> MSMLKREDWYDLTRTTNWTPKYVTENELFPEEMSGARGISMEAWEKYDEPYKITYPEYVSIQREKDSGAYSIKAALERDGFVDRADPGWVSTMQLHFGAIALEEYAASTAEARMARFAKAPGNRNMATFGMMDENRHGQIQLYFPYANVKRSRKWDWAHKAIHTNEWAAIAARSFFDDMMMTRDSVAVSIMLTFAFETGFSNMQFLGLAADAAEAGDHTFASLISSIQTDESRHAQQGGPSLKILVENGKKDEAQQMVDVAIWRSWKLFSVETGPIMDYYTPLESRNQSFKEFMLEWIVAQFERQLLDLGLDKPWYWDQFMQDLDE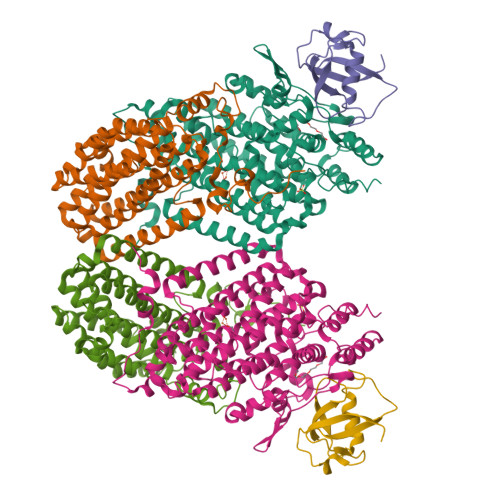THHGMHLGVWYWRPTVWWDPAAGVSPEEREWLEEKYPGWNDTWGQCWDVITDNLVNGKPELTVPETLPTICNMCNLPIAHTPGNKWNVKDYQLEYEGRLYHFGSEADRWCFQIDPERYKNHTNLVDRFLKGEIQPADLAGALMYMSLEPGVMGDDAHDYEWVKAYQKKTNAA;> MSEQQPEALKPLKTWSHLAGNRRRPSEYEVVSTNLHYFTDNPERPWELDSNLPMQTWYKKYCFDSPLKHDDWNAFRDPDQLVYRTYNLLQDGQESYVQGLFDQLNDRGHDQMLTREWVETLARFYTPARYLFHALQMGSVYIHQIAPASTITNCATYETADHLRWLTHTAYRTRELANCYPDVGFGKRERDVWENDPAWQGFRELIEKALIAWDWGEAFTAINLVTKPAVEEALLQQLGSLAQSEGDTLLGLLAQAQKRDAERHRRWSSALVKMALEKEGNREVLQKWVAKWEPLADKAIEAYCSALPDGENAIVEAKSASRYVRQMMGL;> MATFPIMSNFERDFVIQLVPVDTEDTMDQVAEKCAYHSINRRVHPQPEKILRVRRHEDGTLFPRGMIVSDAGLRPTETLDIIFMDN3-(2-aminoquinolin-3-yl)-N-(cyclohexylmethyl)propanamide | C19 H25 N3 O | 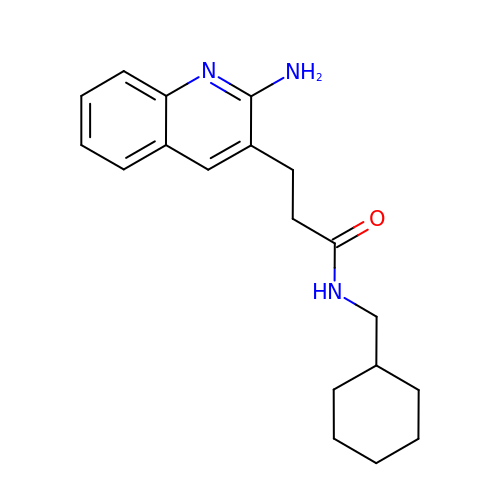YOUIXYWUUXULRM-UHFFFAOYSA-N>EVNGCPPHWKNFTDKCYYFSLEKEIFEDAKLFCEDKSSHLVFINSREEQQWIKKHTVGRESHWIGLTDSEQESEWKWLDGSPVDYKNWKAGQPDNWGSGHGPGEDCAGLIYAGQWNDFQCDEINNFICEKEREAV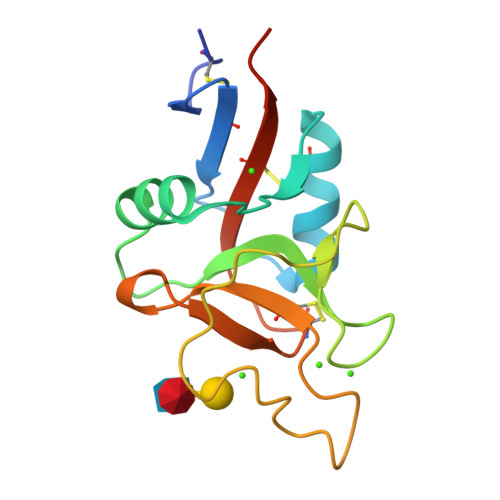PSSIL[4x]> DEELEEIKKETGFSHSQITRLYSRFTSLDKGENGTLSREDFQRIPELAINPLGDRIINAFFPEGEDQVNFRGFMRTLAH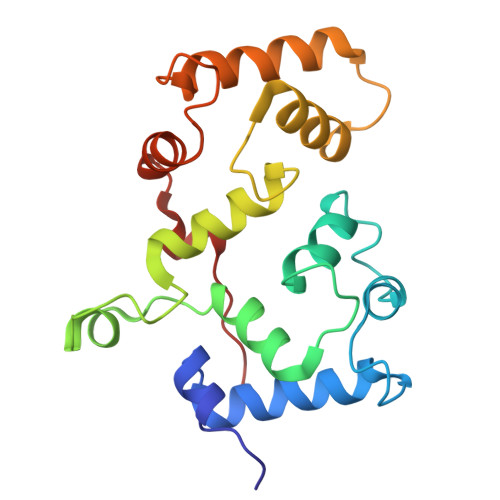FRPIEDNEKSKDVNGPEPLNSRSNKLHFAFRLYDLDKDEKISRDELLQVLRMMVGVNISDEQLGSIADRTIQEADQDGDSAASFTEFVKVLEKVDVEQKMSIRFLH>[5x]SNAMIIRPEQHWFLRLFDWHGSVLSKIIFRLLLNVLMSIIAIISYQWYEQLGIHLTVAPFSLLGIAIAIFLGFRNSAS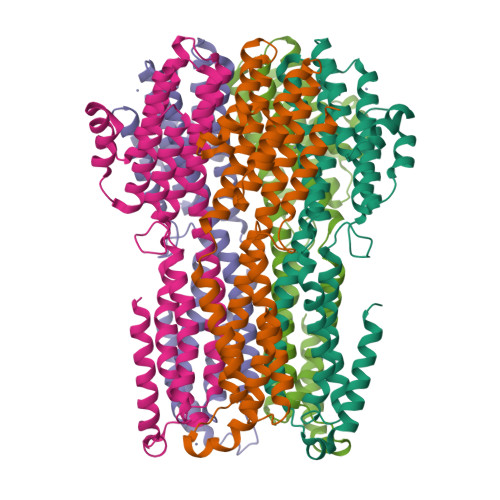YSRFVEARNLWGTVLIAERTLVRQLRNILPAEHDAHRRIVSYLVAFSWSLKHQLRKTDPTADLRRLLPEERVTEILASSMPTNRILLLAGNEIGQLREAGKLSAITYGLMDNKLDELAHVLGGCERLATTPVPFAYTLILQRTVYLFCTLLPFALVGDLHYMTPFVSVFISYTFLSWDSLAEELEDPFGTAANDLPLNAMCNTIERNLLDMTGQHPLPE> MSAKDE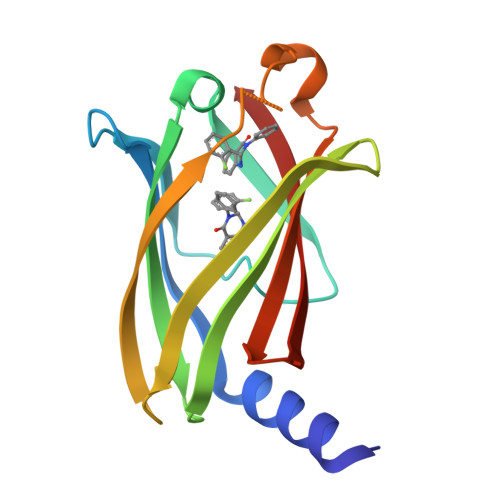RAREILRGFKLNWMNLRDAETGKILWQGTEDLSVPGVEHEARVPKKILKCKAVSRELNFSSTEQMEKFRLEQKVYFKGQCLEEWFFEFGFVIPNSTNTWQSLIEAAPESQMMPASVLTGNVIIETKFFDDDLLVSTSRVRLFYV> NKFITKDDEVIDYIYGKISPLFALQYIRKIDLKHVFEYDYHFEVNGTVVRHKNKGFGYMERFFELKESCDERSKLSKKQYERFNALFNFFEKNGVICMAKDAGTLNTSIEINSLAYHGKYDVMKKFIEEQSVSIEDDYKKAFFLACLGRWEESYDLYSNIILNSIDESNGCVYYLSQINRYRIYQSITQAVTQFNGLGLLTFGRHYKPFTDEFLARIEREMTNFNIDDLFNGMPFEFQKKYKILEFLSDNQFLYDDTVKLFELTNKVRSEMSEGSYSFGMSSDIVVLLRLYDNLRFLYENCLWSVSFHEFHQYIRNSMSLLIEKAEYERTRDIDELGFSFFGKKSGFFMEYYDFVNISRHFKIDDIKNLERSCSIDKIRFGEQEKIEEYLVGIAEEITKQFSANGMNVVFYTQFISEAKAALYFAKYVKLSEEGLGKIVKALLFYFPERDLDIGKRYVWLERLTKCNELPKSIISIIDDFLVLQAEKHIDQNYSEVSSNGLYSRDYGALIKHFEKNFISKRLSEITLCLTQDKQKQIDFL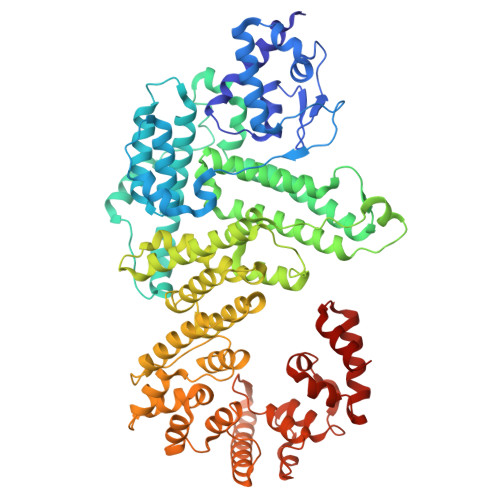FKLLPLLSTNAKSHLLSFKSVENINDLMNGIRIGLIDEFTPEHEELIIEYLETRKVNYIVEKEKGIQTFSSNDYMSTFGIWYFLEEINNSKMEEFIGMDDQYDFFVDPENFDYKKFIPSWLKNYNDKLLGKIAGNKHMKHHVIEVLKERVKNSNDKRYLEILMNYFI>MGSSHHHHHHHHASTGYTSINGKHFYFNTDGIMQIGVFKGPNGFEYFAPANTDANNIEGQAILYQNKFLTLNGKKYYFGSDSKAVTGLRTIDGKKYYFNTNTAVAVTGWQTINGKKYYFNTNTSIASTGYTIISGKHFYFNTDGIMQIGVFKGPDGFEYFAPANTDANNIEGQAIRYQNRFLYLHDNIYYFGNNSKAATGWVTIDGNRYYFEP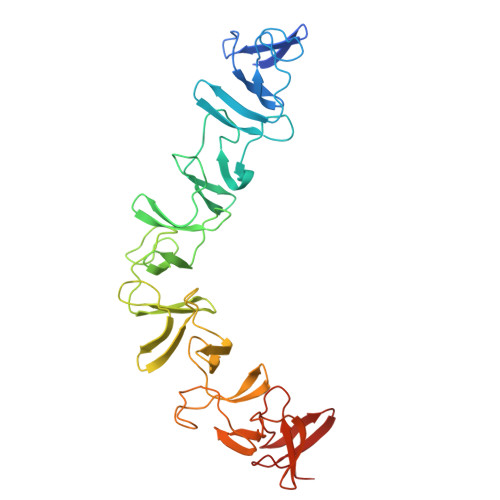NTAMGANGYKTIDNKNFYFRNGLPQIGVFKGSNGFEYFAPANTDANNIEGQAIRYQNRFLHLLGKIYYFGNNSKAVTGWQTINGKVYYFMPDTAMAAAGGLFEIDGVIYFFGVDGVKAP[2x]Inositol pyrophosphates (PP-InsPs) are eukaryotic nutrient messengers. The N-terminal kinase domain of diphosphoinositol pentakisphosphate kinase (PPIP5K) generates the messenger 1,5-InsP8, the C-terminal phosphatase domain catalyzes PP-InsP breakdown. The balance between kinase and phosphatase activities regulates 1,5-InsP8 levels. ScVip1PD is a phytase-like inositol 1-pyrophosphate histidine phosphatase with two conserved catalytic motifs.

Apo crystals of the ScVip1PD initially diffracted to ~3.1 Å. The structure was solved by molecular replacement-single wavelength anomalous diffraction (MR-SAD) on a platinum derivative. In this structure, a large disordered loop (residues 851–918) was located and subsequently replaced by a short Gly-Ser-Ser-Gly linker. The two apo structures of ScVip1PD revealed a conserved histidine acid phosphatase core with two insertion domains. All four molecules in the asymmetric unit of our ScVip1PD crystals display the GAF domain in an “open” conformation. The N-terminus of ScVip1PD (residue 536) and the most C-terminal α9 helix (residues 1079–1094) are well defined by electron density. Plant and human PPIP5Ks contain sequence-diverse linkers of similar length between their kinase and phosphatase domains. An unexpected metal binding site occupied by a Zn2+ ion is formed by His651 and His1064 from the histidine acid phosphatase core, and by Cys793 and His836 from the α-helical insertion domain (see below). The conserved Zn2+ binding site in ScVip1PD positions His836 to form a salt bridge with Asp550, apparently stabilizing the catalytic loop.

>[4x]GAKWVFKGLAIIIRHADRTPKQKFKHSFTSPIFISLLKGHKEEVVIRNVNDLKIVLQALRIALDEKAGNPAKIKVLANALEKKLNFPGTKIQLKPVLNKENEVEKVQFILKWGGEPTHSAKYQATELGEQMRQDFDLLNKSILQNIKIFSSSERRVLHTAQYWTRALFGADELGSDEISIRKDLLDDSNAAKDLMDKVKKKLKPLLREGKEAPPQFAWPSKMPEPYLVIKRVVELMNYHKKIMDNNFAKKDVNSMQTRWCTSEDPSLFKERWDKLFKEFNNAEKVDPSKISELYDTMKYDALHNRQFLENIFDPGLPNEAIADELGSHSLVDRYPINVLAKNNFKIIDSHSMNNSGKNSSNSVGSLGWVLESGKTSTARNPKSSSQFDEPRFMQLRELYKLAKVLFDFICPKEYGISDAEKLDIGLLTSLPLAKQILNDIGDMKNRETPACVAYFTKESHIYTLLNIIYESGIPMRIARNALPELDYLSQITFELYESTDASGQKSHSIRLKMSPGCHTQDPLDVQLDDRHYISCIPKISLTKHLDMDYVQQKLRNKFTRVIMPPKFTPVNITS>HHHHHHFNLPPGNYKKPKLLYCSNGGHFLRILPDGTVDGTRDRSDQHIQFQLSAESVG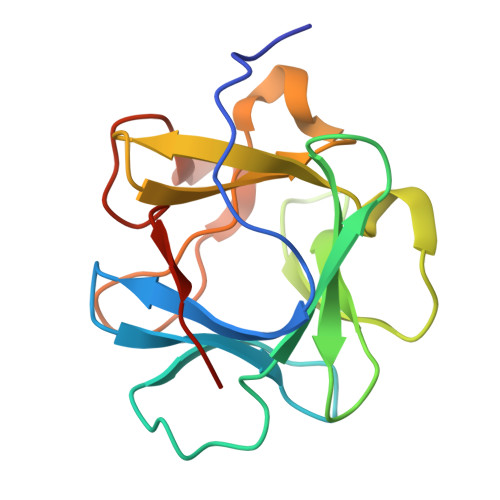EVYIKSTETGQYLAMDTDGLLYGSQTPNEECLFLERLEENHYNTYISKKHAEKNWFVGLKKNGSCKRGPRTHYGQKAILFLPLPVSSD[4x]((2R,3S,4R,5R)-5-(5-AMINO-4-NITRO-1H-IMIDAZOL-1-YL)-3,4-DIHYDROXYTETRAHYDROFURAN-2-YL)METHYL DIHYDROGEN PHOSPHATE | C8 H13 N4 O9 P | 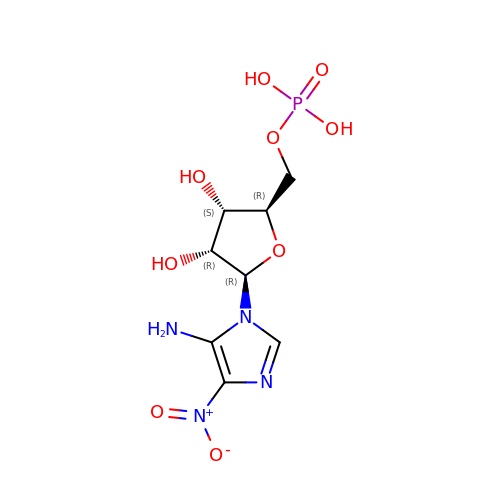YVRCVGZPIYHJLU-AFCXAGJDSA-N>[2x]MRDPFMEALGLKVLHLAPGEAVVAGEVRADHLNLHGTAHGGFLYALADSAFALASNTRGPAVALSCRMDYFRPLGAGARVEARAVEVNLSRRTATYRVEVVSEGKLVALF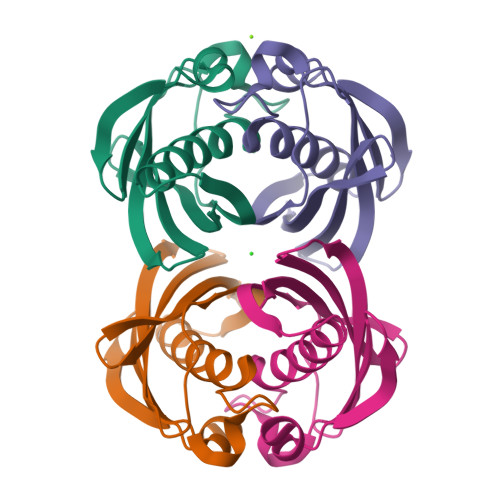TGTVFRLGGDGDDVPAGTGNLAPREA> GIGKFLHA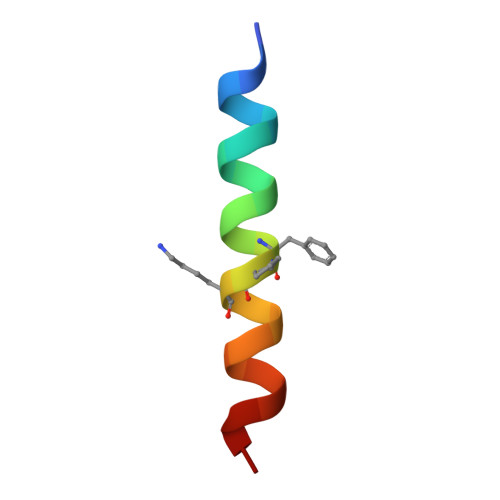AKKFXKAFVAEIMNS>[3x]TETTSFSITKF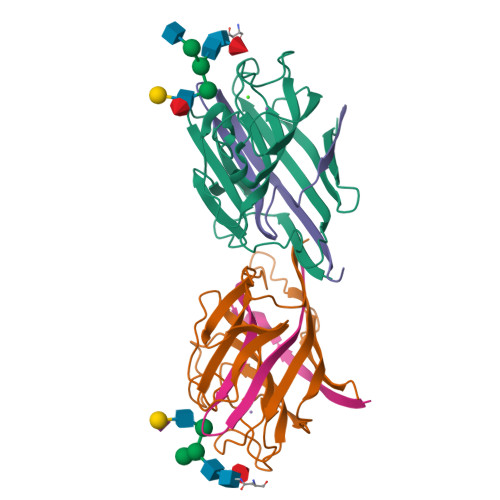GPDQPNLIFQGDGYTTKERLTLTKAVRNTVGRALYSSPIHIWDSKTGNVANFVTSFTFVIDAPNSYNVADGFTFFIAPVDTKPQTGGGYLGVFNSKDYDKTSQTVAVEFDTFYNTAWDPSNGDRHIGIDVNSIKSINTKSWKLQNGKEANVVIAFNGATNVLTVSLTYPN;>[3x]ETSYTLNEVVPLKEFVPEWVRIGFSATTGAEFAAHEVLSWYFNSELSVTSSSN;>[3x]NQ> MLDTNMKTQLKAYLEKLTKPVELIATLDDSAKSAEIKELLAEIAELSDKVTFKEDNSLPVRKPSFLITNPGSNQGPRFAGSPLGHEFTSLVLALLWTGGHPSKEAQSLLEQIRHIDGDFEFETYYSLSCHNCPDVVQALNLMSVLNPRIKHTAIDGGTFQNEITDRNVMGVPAVFVNGKEFGQGRMTLTEIVAKIDTGAEKRAAEELNKRDAYDVLIVGSGPAGAAAAIYSARKGIRTGLMGERFGGQILDTVDIENYISVPKTEGQKLAGALKVHVDEYDVDVIDSQSASKLIPAAVEGGLHQIETASGAVLKARSIIVATGAKWRNMNVPGEDQYRTKGVTYCPHCDGPLFKGKRVAVIGGGNSGVEAAIDLAGIVEHVTLLEFAPEMKADQVLQDKLRSL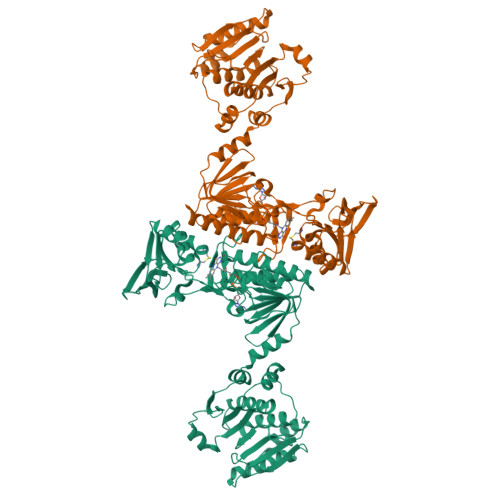KNVDIILNAQTTEVKGDGSKVVGLEYRDRVSGDIHNIELAGIFVQIGLLPNTNWLEGAVERNRMGEIIIDAKCETNVKGVFAAGDCTTVPYKQIIIATGEGAKASLSAFDYLIRTKTA>TVPDRSEVAGKWYIVALASNTDFFLAEKGKMKMVMARISFLGEDELEVSYAAPSPKGCRKWETTFKKTSDDGEVYYSE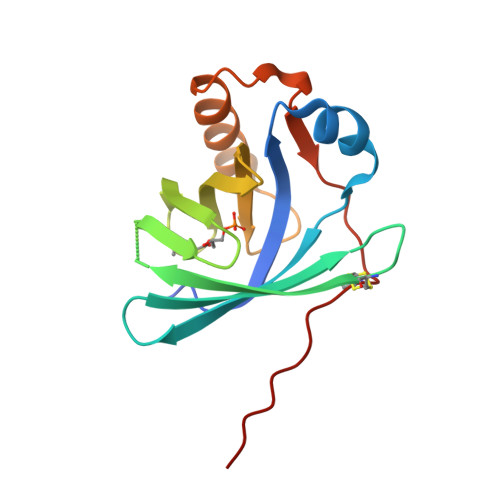EAEKTVEVLDTDYKSYAVIFATRVKDGRTLHMMRLYSRSREVSPTAMAIFRKLARERNYTDEMVAVLPSQAACSVDEVLVPR[2x]> TDFYTIKDAQADLAIAPLNLTVLLAPYSTTPATTLESPTDGSLAIPPGYKSVGHFEKQAGLTLGNEFDSKDIEAYGEPEPIRTIINKRTTTFDFAMYQNQRNVLELIWTQDFSN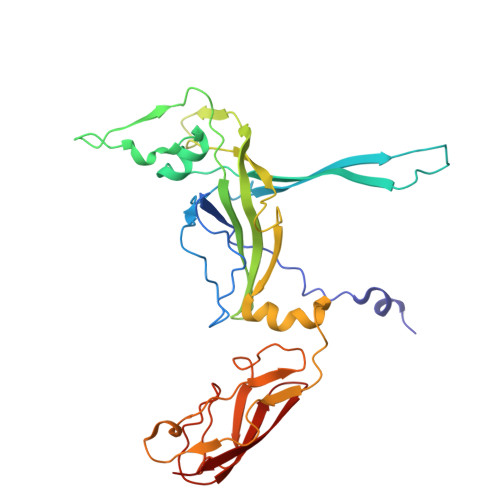IQPSEFGGIVLEAPKVPKNIYYRAILVGMDDRNDRPIWLYWLMPKVKLDKLDNQTLNDDNVIEYKPTLKAFRDDVVGYSVAQGFAGPGWRDLVATAGFGEALTALTITPGSPTVTVATGASHTAQLLVEGDNGINYTPDVVFTSSAPDKASVSAAGLVTGVAAGSATITATKGALTATATVTVTA> TEMSVRKIAAHMKSNPNAKVIFMVGAGISTSCGIPDFRSPGTGLYHNLARLKLPYPEAVFDVDFFQSDPLPFYTLAKELYPGNFRPSKFHYLLKLFQDKDVLKRVYTQNIDTLERQAGVKDDLIIEAHGSFAHCHCIGCGKVYPPQVFK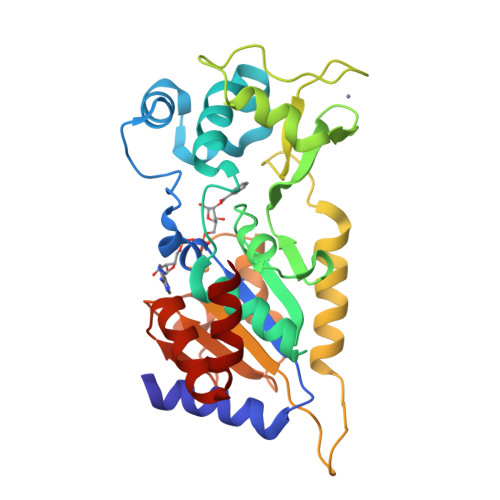SKLAEHPIKDFVKCDVCGELVKPAIVFFGEDLPDSFSETWLNDSEWLREKITTSGKHPQQPLVIVVGTSLAVYPFASLPEEIPRKVKRVLCNLETVGDFKANKRPTDLIVHQYSDEFAEQLVEELGWQEDFEKILTAQ>GSFTMDDISPSELKTILHSKRANLYYLQHCRVLVNGGRVEYVTDEGRHSHYWNIPIANTTSLLLGTGTSITQAAMRELARAGVLVGFCGGGGTPLFSANEVDVE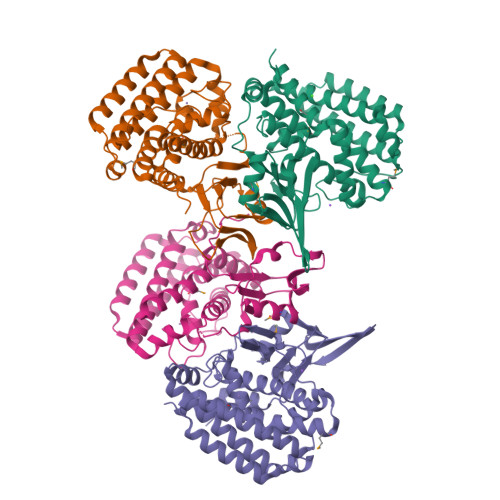VSWLTPQSEYRPTEYLQRWVGFWFDEEKRLVAARHFQRARLERIRHSWLEDRVLRDAGFAVDATALAVAVEDSARALEQAPNHEHLLTEEARLSKRLFKLAAQATRYGEFVRAKRGSGGDPANRFLDHGNYLAYGLAATATWVLGIPHGLAVLHGKTRRGGLVFDVADLIKDSLILPQAFLSAMRGDEEQDFRQACLDNLSRAQALDFMIDTLKDVAQRSTVSA[4x]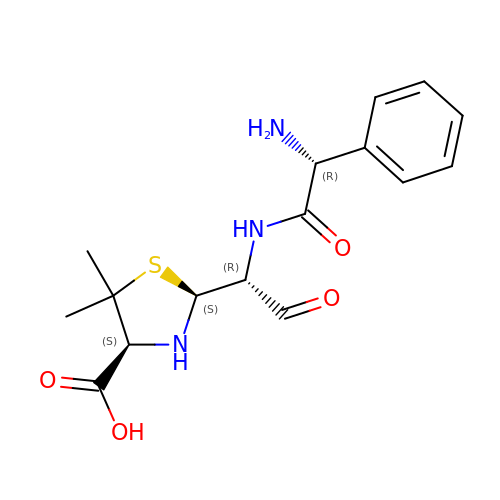(2S,4S)-2-[(1R)-1-{[(2R)-2-amino-2-phenylacetyl]amino}-2-oxoethyl]-5,5-dimethyl-1,3-thiazolidine-4-carboxylic acid | C16 H21 N3 O4 S | WHAIWIUXAXKSOT-NMKXLXIOSA-N> GLVPRGSHMNVLVIEDDKVFRGLLEEYLSMKGIKVESAERGKEAYKLLSEKHFNVVLLDLLLPDVNGLEILKWIKERSPETEVIVITGHGTIKTAVEAMKMGAYDFLTKPCMLEEIELTINKAIEHRKLRKENELLRREKDL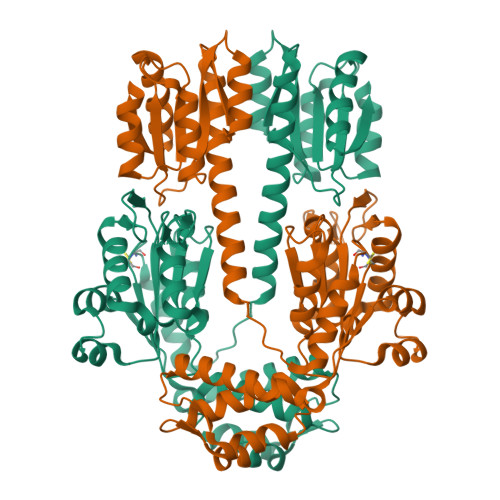KEEEYVFESPKMKEILEKIKKISCAECPVLITGESGVGKEVVARLIHKSSDRSKEPFVALNVASIPRDIFEAELFGYEKGAFTGAVSSKEGFFELADGGTLFLDEIGELSLEAQAKLLRVIESGKFYRLGGRKEIEVNVRILAATNRNIKELVKEGKFREDLYYRLGVIEIEIPPLRERKEDIIPLANHFLKKFSRKYAKEVEGFTKSAQELLLSYPWYGNVRELKNVIERAVLFSEGKFIDRGELSCLVNSKGIKNKHKSIKEIEKEEIIKVLKEVNFNKKLASEILGIPLRTLYRRLKEYGIE>GHHHHHHAMSMQDTLLTLDTPAAVIDLDRMQRNIARMQQRMDAQGVRLRPHVKTSKSVPVAAAQRAAGASGITVSTLKEAEQFFAAGTTDILYAVSMAPHRLPQALQLRRRGCDLKLIVDSVAAAQAIAAFGREQGEAFEVWIEIDTDGHRSGVGADDTPLLLAIGRTLHDGGMRLGGVLTHAGSSYELDTPEALQALAERERAGCVQAAEALRAAGLPCPVVSVGSTPTALAASRLDGVTEVRAGVYVFFDLVMRNIGVCAAEDVALSVLATVIGHQADKGWAIVDAGWMAMSRDRGTARQKQDFGYGQVCDLQGRVMPGFVLTGANQEHGILARADGAAEADIATRFPLGTRLRILPNAACATGAQFPAYQALAADGSVQT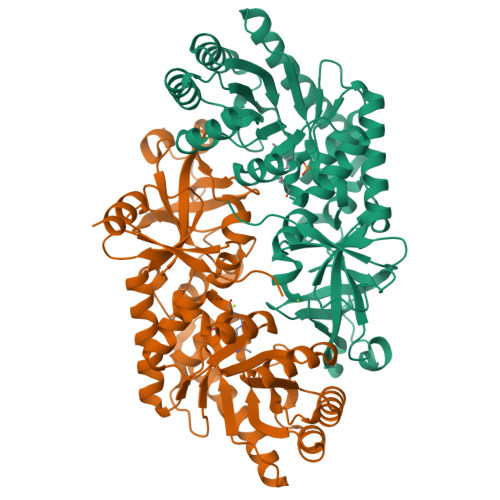WERLHGW[2x]>[6x]GSEELLDLFNRQVTQE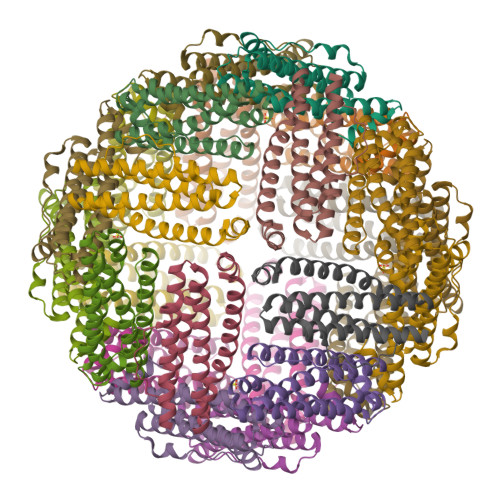FTASQVYLSASIWFDQNDWEGMAAYMLAESAEEREHGLGFVDFANKRNIPIELQAVPAPVSCAEWSSPEDVWQSILELEQANTRSLLNLAEAASTCHDFAVMAFLNPFHLQQVNEEDKIGSILAKVTDENRTPGLLRSLDVVSFLGPCLFRS> SNAKDVPDSQQHPAPEKSSKVSEQLKCCSGILKEMFAKKHAAYAWPFYKPVDVEALGLHDYCDIIKHPMDMST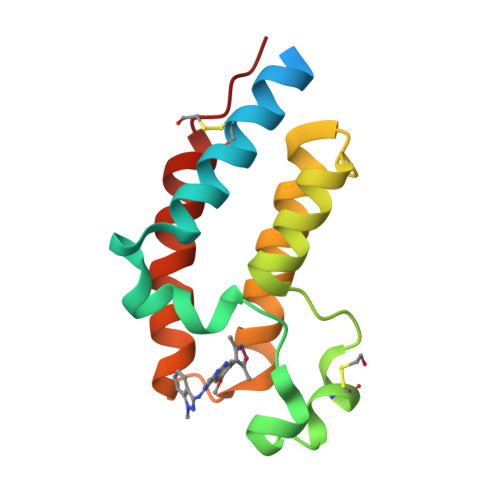IKSKLEAREYRDAQEFGADVRLMFSNCYKYNPPDHEVVAMARKLQDVFEMRFAKMPDE>[2x]MEYTQLGRIGLKVSRLVLGTMNFGPTTDEAESHAIMDAALDAGINFFDTANVYGWGENKGRTEEILGSWFAQGGDRRDKVVLATKVYGNMGLDGPAWPNHDKLSALNIRRSVDASLKRLGTDHIDLYQFHHVDRDTPWDEIWQAMDVLVRQGKILYVG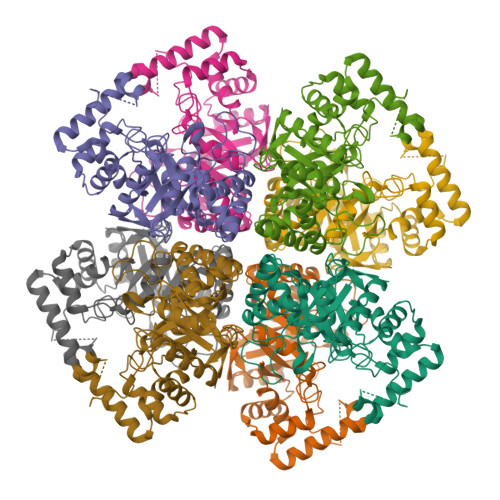SSNFAGWNIAQANETAARHGRLGLVSEQCLYNLCERRAEMEVVPAAREYGLGVIAWSPLHGGLLGGAIRKEQEGGNRRAASGRAADALKDPQQREQIQRYEDLLDKHGLEPGEVALAWLLTRPGVTGPIVGPRTADQLASAVRAAELTLTDEVLTALDEIFPGPGPSPEAFAW> GPNLELLESFGQNYPEEADGTLDCISMALTCTFNRWGTLLAVGCNDGRIVIWDFLTRGIAKIISAHIHPVCSLCWSRDGHKLVSASTDNIVSQWDVLSGDCDQRFRFPSPILKVQYHPRDQNKVLVCPMKSAPVMLTLSDSKHVVLPVDDDSDLNVVASFDRRGEYIYTGNAKGKILVLKTDSQDLVASFRVTTGTS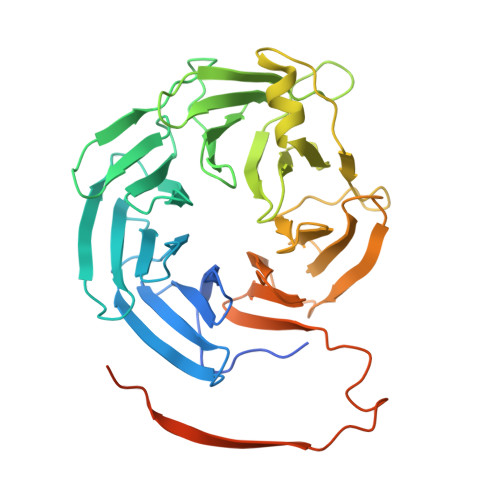NTTAIKSIEFARKGSCFLINTADRIIRVYDGREILTCGRDGEPEPMQKLQDLVNRTPWKKCCFSGDGEYIVAGSARQHALYIWEKSIGNLVKILHGTRGELLLDVAWHPVRPIIASISSGVVSIWAQNQVENWSAFAPDFKELDENVEYEERESEFDIEDEDKSEPKQTGADAAEDEEVDVTSV> MEKLAASTEPQGPRPVL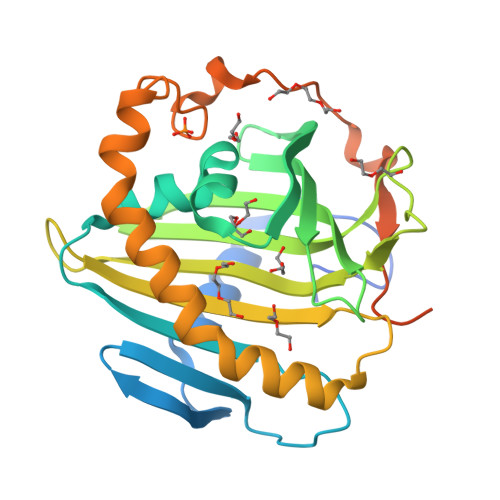GRESVQVPDDQDFRSFRSECEAEVGWNLTYSRAGVSVWVQAVEMDRTLHKIKCRMECCDVPAETLYDVLHDIEYRKKWDSNVIETFDIARLTVNADVGYYSWRCPKPLKNRDVITLRSWLPMGADYIIMNYSVKHPKYPPRKDLVRAVSIQTGYLIQSTGPKSCVITYLAQVDPKGSLPKWVVNKSSQFLAPKAMKKMYKACLKYPEWKQKHLPHFKPWLHPEQSPLPSLALSELSVQHADSLENIDESAVAESREERMGGAGGEGSDDDTSLT> MKTIYNFKQRIKEDPEYIRKAHELTLNTTKPKAGLKGTYGLLGSKEWWDNLENGSIPQKEI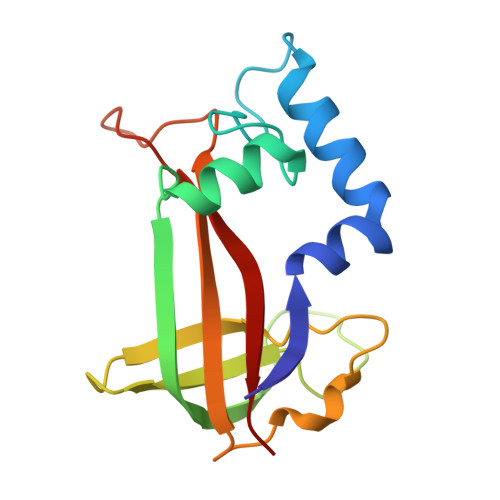SGTIKKVYLTGQDNTEDFNTIDIETENKTLCTEGTYTNKNTDRKHYEAGKKITIKYAFDPLKKPKPNGDIDYSKIVVEILISE>[2x]MQKIGILGAMREEITPILELFGVDFEEIPLGGNVFHKGVYHNKEIIVAYSKIGKVHS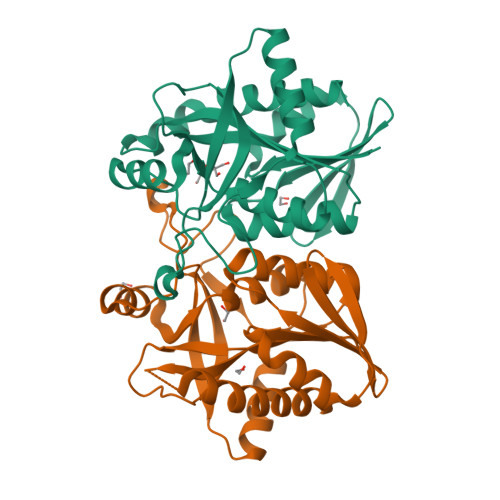TLTTTSMILAFGVQKVLFSGVAGSLVKDLKINDLLVATQLVQHDVDLSAFDHPLGFIPESAIFIETSGSLNALAKKIANEQHIALKEGVIASGDQFVHSKERKEFLVSEFKASAVEMEGASVAFVCQKFGVPCCVLRSISDNADEKAGMSFDEFLEKSAHTSAKFLKSMVDEL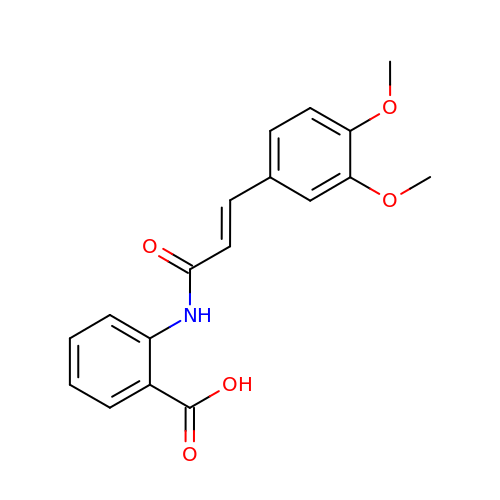2-{[(2E)-3-(3,4-dimethoxyphenyl)prop-2-enoyl]amino}benzoic acid | C18 H17 N O5 | NZHGWWWHIYHZNX-CSKARUKUSA-N>MIIGYFDGLCEPKNPGGIATFGFVIYLDNRKIEGYGLAEKPFSINSTNNVAEYSGLICLMETMLRLGISSPIIKGDSQLVIKQMNGEYKVKAKRIIPLYEKAIELKKKLNATLIWVPREENKEADRLSRVAYELVRRGKLRDI[2x]

Ribonuclease HI from the hyperthermophile Sulfolobus tokodaii (Sto-RNase HI) is a monomeric protein of 149 amino acids. Sto-RNase HI is highly stable, and is stabilized through the C-terminal tail. The C-terminus of Sto-RNase HI is anchored to the core region by one disulfide bond (Cys58-Cys145), several hydrogen bonds, and hydrophobic interactions. The C-terminal residues of Sto-RNase HI contribute to stability through local hydrogen bonds, hydrophobic interactions, and a disulfide bond.

First, we investigated in detail the stabilization effect of the Sto-RNase HI C-terminus, by measuring the stability of a C58/145A variant lacking the disulfide bond, and a ΔC6 variant lacking the six C-terminal residues. The shape of the spectra was almost the same for the wild-type and variant proteins. The crystal structure of ΔC6 Sto-RNase HI was solved at a resolution of 1.66 Å, as shown in Figure 2B. Two molecules are contained per asymmetric unit. The root-mean-square deviations of the Cα atoms for the A and B chains of the ΔC6 variant against the wild-type protein were 0.446 and 0.436Å. C-terminal residues 142 and 143 of ΔC6 Sto-RNase HI were not observed because of disorder, indicating that deletion of the previous C-terminal residues made the new C-terminus flexible. The denaturation temperature is 102°C for the wild-type, 93°C for C58/145A and 78°C for ΔC6 Sto-RNase HI. These results indicated that Sto-RNase HI is a hyperthermostable protein with a denaturation temperature beyond the boiling temperature, and is destabilized by 9°C by elimination of the disulfide bond and by 24°C by C-terminal truncation. In contrast, the ΔC6 variant shifted the curve downward and flattened it. This is the result of decreases in ΔH and ΔCp. Because the C-terminal truncation eliminates hydrogen bonds and hydrophobic interactions, this result suggested that elimination of these forces at the C-terminal region was mainly responsible for the decreases in ΔH and ΔCp, resulting in the destabilization of ΔC6 Sto-RNase HI.> MGSSHHHHHHSSGLVPAGSHMASQSSKKEKKTKPNVIIILADDLGYGDLECYGTTRVHTPNVNRLASEGIRFTNVHATASTSTPSRYALLTGEYAWRKKGTGVAAGNAGMIIRPEQYTIADMFKSADYTTGAIGKWHLGLGDKTGTQDWNGTISPALKDIGFDYSYIMAATADRVPCIYIENGKVADYDSTAPIEVSYQKPFEGEPTGRKNPELLYNLKPSHGHDMAIVNGISRIGYMKGGGKALWKDENIADTITSHAIRFIEENKERPFFLYFATNDVHVPRFPHERFRGKNPMGLRGDAIVQFDWSVGEIMKTLDRLGLTENTLIILSSDNG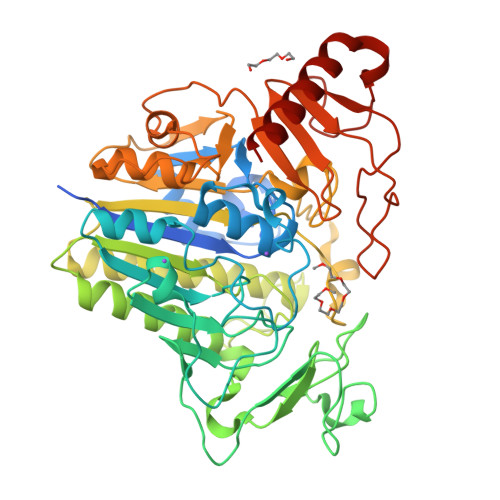PVLDDGYDDKAVELAGSHKPGGPFRGGKYSAFEAGTCVPAIVRYPAQVKKNQTLNTLLSQIDWIQSLASLVNVTIPQSKAPDSQNHLDSWLGKSKKDRPWVIEESNILALSVRKGKWKYIEPSNGSPMITWGPKIETGYAPYDQLFDMNKSEFESENLAPKYPAIVKEMKDILVQERAKGKK> MSEKRVQPLARDAMAYVLAGGRGSRLKELTDRRAKPAVYFGGKARIIDFALSNALNSGIRRIGVATQYKAHSLIRHLQRGWDFFRPERNESFDILPASQRVSETQWYEGTADAVYQNIDIIEPYAPEYMVILAGDHIYKMDYEYMLQQHVDSGADVTIGCLE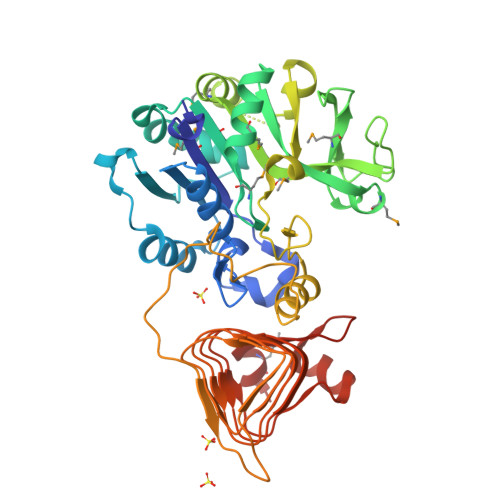VPRMEATGFGVMHVNEKDEIIDFIEKPADPPGIPGNEGFALASMGIYVFHTKFLMEAVRRDAADPTSSRDFGKDIIPYIVEHGKAVAHRFADSCVRSDFEHEPYWRDVGTIDAYWQANIDLTDVVPDLDIYDKSWPIWTYAEITPPAKFVHDDEDRRGSAVSSVVSGDCIISGAALNRSLLFTGVRANSYSRLENAVVLPSVKIGRHAQLSNVVIDHGVVIPEGLIVGEDPELDAKRFRRTESGICLITQSMIDKLDL>[2x]SDKII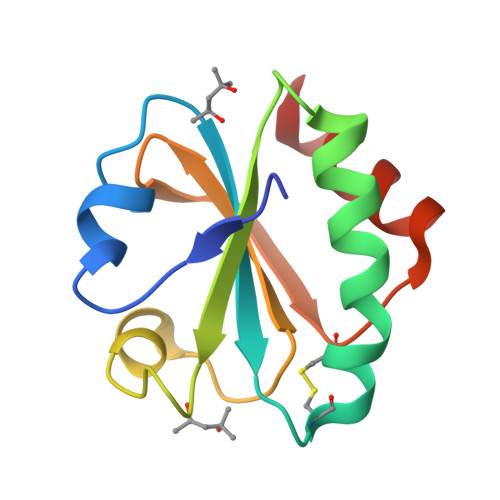HLTEDSFDTDVLKADGAILVDFWAEWCGPCKMIAPILDEIADEYQGKLTVAKLNIDQNPGTAPKYGIRGIPTLLLFKNGEVAATKVGALSKGQLKEFLDANLA>MSSTPSNQNIIPIIKK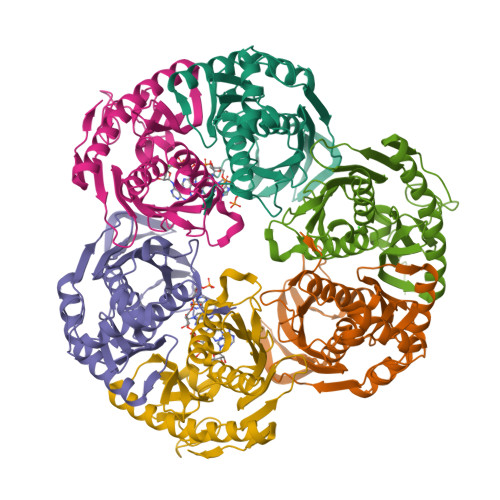ESIVSLFEKGIRQDGRKLTDYRPLSITLDYAKKADGSALVKLGTTMVLAGTKLEIDKPYEDTPNQGNLIVNVELLPLAYETFEPGPPDENAIELARVVDRSLRDSKALDLTKLVIEPGKSVWTVWLDVYVLDYGGNVLDACTLASVAALYNTKVYKVEQHSNGISVNKNEVVGKLPLNYPVVTISVAKVDKYLVVDPDLDEESIMDAKISFSYTPDLKIVGIQKSGKGSMSLQDIDQAENTARSTAVKLLEELKKHLGI[12x];>MREMLQVERPKLILDDGKRTDGRKPDELRSIKIELGVLKNADGSAIFEMGNTKAIAAVYGPKEMHPRHLSLPDRAVLRVRYHMTPFSTDERKNPAPSRREIELSKVIREALESAVLVELFPRTAIDVFTEILQADAGSRLVSLMAASLALADAGIPMRDLIAGVAVGKADGVIILDLNETEDMWGEADMPIAMMPSLNQVTLFQLNGSMTPDEFRQAFDLAVKGINIIYNLEREALKSKYVEFKEEGV[12x]>[2x]MNGDCVDAKRVDTTDASKDGASASQPMQVDAKPQSHAFRYSLNYPNIGHCIIINNKNFDRRTGMNPRNGTDVDAGNVMNVFRKLGYIVKVYNDQTVAQIMQVLTTVAHDDHSRCASLVCVLLSHGDEGVFFGTDTSVDLKSLTSLFRGDRCPSLVGKPKLFFIQACRGTELDPGVETD;>[2x]RERIPVEADFLYAYSTVPGYYSWRTTMTGSWFIQSLCEMMTKYGSELELLQIMTRVNHKVALDFESTSNMPGFDAKKQIPCIVSMLTKEMYFTPLEHHHHHH;> DEVD

Caspase (or cysteinyl-aspartate specific proteases) enzymes play important roles in apoptosis and inflammation, and the non-identical but overlapping specificity profiles (that is, cleavage recognition sequence) direct cells to different fates. Although all caspases prefer aspartate at the P1 position of the substrate, the caspase-6 subfamily shows preference for valine at the P4 position, while caspase-3 shows preference for aspartate. Zebrafish have two copies of the caspase-3 gene, called DrCasp-3a and DrCasp-3b. In comparison with human caspases, caspase-3a from zebrafish has relaxed specificity and demonstrates equal selection for either valine or aspartate at the P4 position.

We first examined changes at CP-N162 by mutating the residue to Val or Thr in DrCasp-3a or to Val, Thr, or Glu in HsCasp-3. CP-N162 forms a hydrogen bond with the carboxylate of the P4 aspartate in caspase-3. In addition, the smaller side-chain of CP-T162 could potentially hydrogen bond with the carboxylate of the P4 aspartate, or it could increase hydrophobicity of the S4 binding pocket, depending on the orientation of the side-chain hydroxyl or methyl groups. The rationale for CP-T162 and CP-V162 was to determine whether increasing hydrophobicity in the S4 subsite would result in changes in substrate selection. In contrast, the CP-N162 to Thr variant of DrCasp-3a demonstrated no activity against VEID substrate. In addition, the activity of CP-N162T against DEVD was approximately ten-fold lower than that of the wild-type enzyme, due primarily to a decrease in kcat. We determined the X-ray crystal structure of DrCasp-3a(CP-N162T) variant at 2.7 Å resolution, and the data showed little to no change in the active site. The hydroxyl group of the Thr side-chain forms a hydrogen bond with its backbone amide group, which presumably stabilizes the turn in active site loop 3 (called L3). The methyl group of the Thr side-chain is oriented toward the acetyl group of the substrate, while the P4 aspartate forms three hydrogen bonds with groups in the L3 and L4 loops. Thus, it is not clear from the structure why this variant has no activity against VEID substrate and a lower catalytic efficiency against DEVD substrate.>GSHMEEIKCLLCRYLKERQEKFISDWKKKVIIRERDPYKEEIIKNGEHLLSA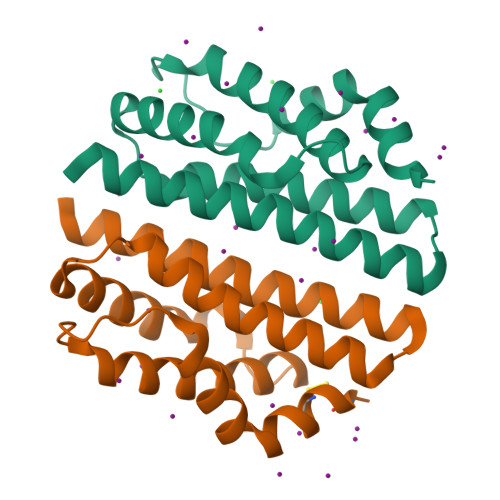FIMYLKEEISLQEIEITSKKIARERIDAKVNIAEFIHNTNVAKIEIMNILTLLNPDLQQYQALVKKINQFFDHLIYYTVHSYYEQKA[2x]>MSLKQQFSTKAFQAANLEAYKAQMKEMEESFGALL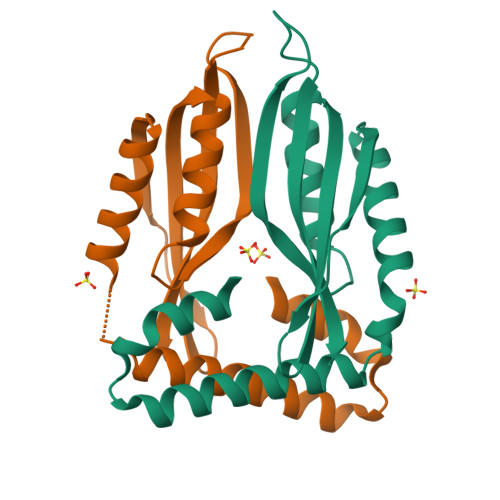RQLPSDTEVPGLLEDITRTGLGSGLEFEEIKLLPEVAQQFYIELPIQISVVGGYHDLATFVSGVSSLPRIVTLHDFEIKPVAPGSTSKLRMSILAKTYRYNDKGEGHHHHHH[2x]> STRFTEEYQLFEELGKGAFSVVRRCVKVLAGQEYAAKIINTKKLSARDHQKLEREARICRLLKHPNIVRLHDSISEEGHHYLIFDLVTGGELFEDIVAREYYSEADASHCIQQILEAVLHCHQMGVVHRDLKPENLLLASKLKGAAVKLADFGLAIEVEGEQQAWFGFAGTPGYLSPEVLRKDPYGKPVDLWACGVILYILLVGYPPFWDEDQHRLYQQIKAGAYDFPSPE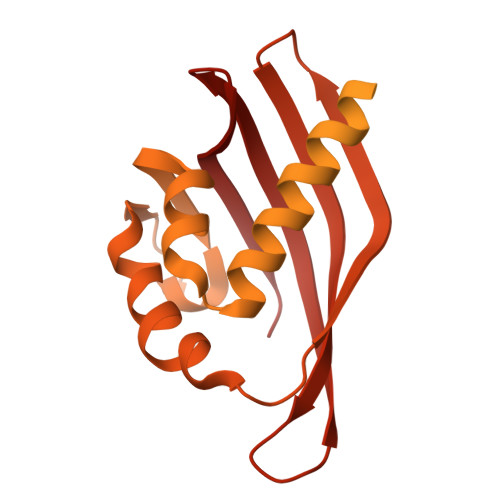WDTVTPEAKDLINKMLTINPSKRITAAEALKHPWISHRSTVASCMHRQETVDCLKKFNARRKLKGAILTTMLATRNFSGGKSGGNKKSDGVKESSESTNTTIEDEDTKVRKQEIIKVTEQLIEAISNGDFESYTKMCDPGMTAFEPEALGNLVEGLDFHRFYFENLWSRNSKPVHTTILNPHIHLMGDESACIAYIRITQYLDAGGIPRTAQSEETRVWHRRDGKWQIVHFHRSGAPSVLPH The metazoan tRNA ligase complex (tRNA-LC) has essential roles in tRNA biogenesis and unfolded protein response. Its catalytic subunit RTCB contains a conserved active-site cysteine that is susceptible to metal ion-induced oxidative inactivation. To preserve the function of RTCB under aerobic conditions, the tRNA-LC relies on the flavin adenine dinucleotide (FAD)-containing oxidoreductase PYROXD1 to protect its catalytic center from oxidation. Here, we report a cryogenic electron microscopic structure of the human RTCB–PYROXD1 complex, revealing that PYROXD1 directly interacts with the catalytic center of RTCB through its carboxy-terminal tail.

To visualize the interaction between RTCB and PYROXD1, we reconstituted the RTCB–PYROXD1 complex in the presence of NADH and Mg2+ ions and analyzed it using single-particle cryo-EM. To overcome the orientation bias of the particles, two datasets were acquired using samples prepared in the presence and absence of octyl-beta-glucoside and combined to yield a molecular reconstruction of the RTCB–PYROXD1 complex at a resolution of 3.3 Å. The resulting model comprises a single molecule of RTCB and PYROXD1, indicating that RTCB and PYROXD1 interact with a 1:1 stoichiometry. The interaction involves the C-terminal domain (CTD) of PYROXD1, whose function has hitherto remained unclear, and the active-site cleft of RTCB, spanning an extensive interface with a buried surface area of 1,715 Å2. The molecular reconstruction shows clear densities for the nicotinamide and flavin dinucleotides within the active center of PYROXD1. Based on the kinetics of NADH oxidation and the dependence of RTCB–PYROXD1 interaction on NAD(P)H, we infer that the PYROXD1 is in the CTC state (that is, bound to NAD+–FADH−) when it interacts with RTCB. As in other flavoprotein oxidoreductases22–27, the ligands are positioned by PYROXD1 such that the flavin ring of the FADH− molecule stacks with the nicotinamide ring of NAD+, forming a π–π interaction. The structure of the RTCB–PYROXD1 complex reveals that the PYROXD1 CTD engages with the catalytic cleft of RTCB, thereby blocking the substrate binding sites and rendering the catalytic center inaccessible. The C-terminal tail is structurally disordered in free PYROXD1 but adopts an alpha-helical conformation upon interaction with RTCB, as it inserts into the catalytic center of RTCB and forms hydrophobic interactions with RTCB through Ile493, Ile495, Tyr498 and Phe499 of PYROXD1. Furthermore, the C-terminal helix of PYROXD1 contacts RTCB by hydrogen bonding interactions of the C-terminal carboxylate group with the backbone amide group of Phe118 of RTCB, while the side chain of the C-terminal residue (Asp500 of PYROXD1) coordinates one of the two Mg2+ ions (position B) in the RTCB catalytic center.

> SNAMSRSYNDELQFLEKINKNCWRIKKGFVPNMQVEGVFYVNDALEKLMFEELRNACRGGGVGGFLPAMKQIGNVAALPGIVHRSIGLPDVHSGYGFAIGNMAAFDMNDPEAVVSPGGVGFDINCGVRLLRTNLDESDVQPVKEQLAQAMFDHIPVGVGSKGVIPMNAKDLEEALEMGVDWSLREGYAWAEDKEHCEEYGRMLQADPNKVSARAKKRGLPQLGTLGAGNHYAEIQVVDEIFNEYAAKKMGIDHKGQVCVMIHSGSRGLGHQVATDALVAMEKAMKRDKIIVNDRQLACARIASPEGQDYLKGMAAAGNYAWVNRSSMTFLTRQAFAKVFNTTPDDLDLHVIYDVSHNIAKVEQHVVDGKERTLLVHRKGSTRAFPPHHPLIAVDYQLTGQPVLIGGTMGTCSYVLTGTEQGMTETFGTTCHGAGRALSRAKSRRNLDFQDVLDKLADMGIAIRVASPKLVMEEAPESYKNVTDVVNTCHDAGISKKAIKLRPIAVIKG;> GPMEAARPPPTAGKFVVVGGGIAGVTCAEQLATHFPSEDILLVTASPVIKAVTNFKQISKILEEFDVEEQSSTMLGKRFPNIKVIESGVKQLKSEEHCIVTEDGNQHVYKKLCLCAGAKPKLICEGNPYVLGIRDTDSAQEFQKQLTKAKRIMIIGNGGIALELVYEIEGCEVIWAIKDKAIGNTFFDAGAAEFLTSKLIAEKSEAKIAHKRTRYTTEGRKKEARSKSKADNVGSALGPDWHEGLNLKGTKEFSHKIHLETMCEVKKIYLQDEFRILKKKSFTFPRDHKSVTADTEMWPVYVELTNEKIYGCDFIVSATGVTPNVEPFLHGNSFDLGEDGGLKVDDHMHTSLPDIYAAGDICTTSWQLSPVWQQMRLWTQARQMGWYAAKCMAAASSGDSIDMDFSFELFAHVTKFFNYKVVLLGKYNAQGLGSDHELMLRCTKGREYIKVVMQNGRMMGAVLIGETDLEETFENLILNQMNLSSYGEDLLDPNIDIEDYFD>[2x]KETNQKPYKETYG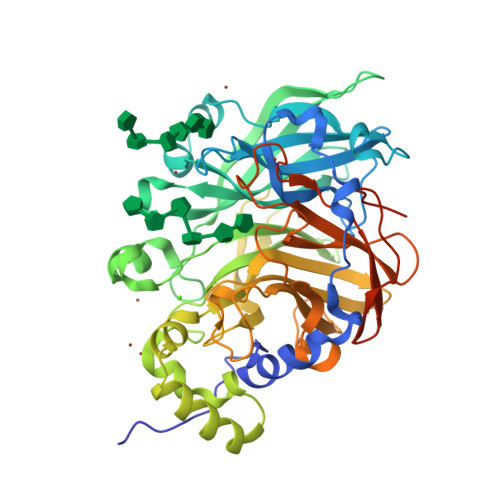ISHITRHDMLQIPEQQKNEKYQVPEFDSSTIKNISSAKGLDVWASWPLQNADGTVANYHGYHIVFALAGDPKNADDTSIYMFYQKVGETSIDSWKNAGRVFKDSDKFDANDSILKDQTQEWSGSATFTSDGKIRLFYTDFSGKHYGKQTLTTAQVNVSASDSSLNINGVEDYKSIFDGDGKTYQNVQQFIDEGNYSSGDNHTLRDPHYVEDKGHKYLVFEANTGTEDGYQGEESLFNKAYYGKSTSFFRQESQKLLQSDKKRTAELANGALGMIELNDDYTLKKVMKPLIASNTVTDEIARANVFKMNGKWYLFTDSRGSKMTIDGITSNDIYMLGYVSNSLTGPYKPLNKTGLVLKMDLDPNDVTFTYSHFAVPQAKGNNVVITSYMTNRGFYADKQSTFAPSFLLNIKGKKTSVVKDSILEQGQLTVNKTDPNSSSVDKLAAALEHHHHHH> MKVHEIPRSQLLKIKQYEGSFVEWYRDLQEDRKKFASLLFRWAAFGYAAREDDGATYISPSQALLERRLLLGDAEDVAIKFLDVLFKGGAPSSSCYSLFYEDFALRDKAKYSGAKREFIEGLATMPLDKIIERIRQDEQLSKIPAEEWLILGAEYSPEEIWEQVAPRIVNVDRSLGKQLRERLGIKCRRPHDAGYCKILMEVVARQLRSHNETYHEYLNQTHEMKTKVANNLTNEFDLVCEFAEVLEEKNYGLGWYVLWQGVKQALKEQKKPTKIQIAVDQLRQPKFAGLLTAKWRALKGAYDTWKLKKRLEKRKAFPYMPNWDNDYQIPVGLTGLGVF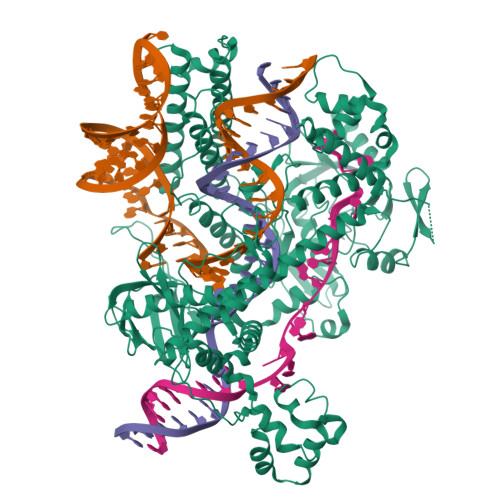TLEVKRTEVVVDLKEHGKLFCSHSHYFGDLTAEKHPSRYHLKFRHKLKLRKRDSRVEPTIGPWIEAALREITIQKKPNGVFYLGLPYALSHGIDNFQIAKRFFSAAKPDKEVINGLPSEMVVGAAALNLSNIVAPVKARIGKGLEGPLHALDYGYGELIDGPKILTPDGPRCGELISLKRDIVEIKSAIKEFKACQREGLTMSEETTTWLSEVESPSDSPRCMIQSRIADTSRRLNSFKYQMNKEGYQDLAEALRLLDAMDSYNSLLESYQRMHLSPGEQSPKEAKFDTKRASFRDLLRRRVAHTIVEYFDDCDIVFFEDLDGPSDSDSRNNALVKLLSPRTLLLYIRQALEKRGIGMVEVAKDGTSQNNPISGHVGWRNKQNKSEIYFYEDKELLVMDADEVGAMNILCRGLNHSVCPYSFVTKAPEKKNDEKKEGDYGKRVKRFLKDRYGSSNVRFLVASMGFVTVTTKRPKDALVGKRLYYHGGELVTHDLHNRMKDEIKYLVEKEVLARRVSLSDSTIKSYKSFAHV>[2x]MINKDSLTHHISQQFNAELEDVRSHLLAMGGLVEKQVNDAVNALIDADSGLAQQVREIDDQINQMERNIDEECVRILARRQ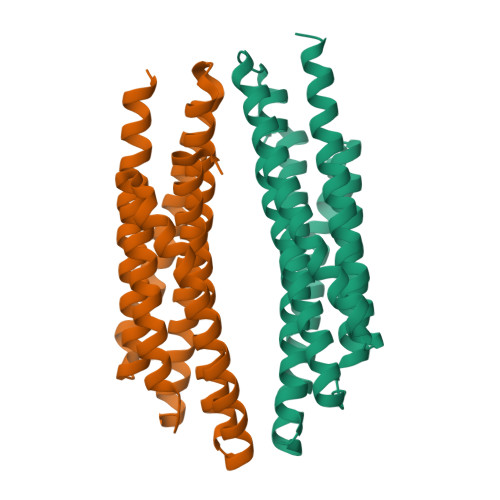PAASDLRLIISISKSVIDLERIGDEASKVARRAIQLCEEGESPRGYVEVRHIGSQVQKMVQEALDAFARFDADLALSVAQYDKTVDREYKTALRELVTYMMEDPRAISRVLNIIWALRSLERIGDHARNIAELVIYLVRGTDVRHIGLTRMKEEVENNRGELEHHHHHH> GSHMFSLITWNIDGLDLNNLSERARGVCSYLALYSPDVIFLQEVIPPYYSYLKKRSSNYEIITGHEEGYFTAIMLKKSRVKLKSQEIIPFPSTKMMRNLLCVHVNVSGNELCLMTSHLESTRGHAAERMNQLKMVLKKMQEAPESATVIFAGDTNLRDREVTRSGGLPNNIVDVWEFLGKPKHCQYTWDTQMNSNLGITAACKLRFDRIFFRAAAEEGHIIPRSLDLLGLEKLDCGRFPSDHWGLLCNLDIIL

Tyrosyl-DNA phosphodiesterase 2 (TDP2) {also known as TRAF and TNF receptor-associated gene (TTRAP) or ETS1-associated protein II (EAPII) } is a 5′-tyrosyl DNA phosphodiesterase that can remove the covalently-attached abortive complexes generated by DNA topoisomerase II (TOP2) when it is unable to complete its normal catalytic cycle. Fortunately, this type of DNA lesion is efficiently repaired, in part though the action of TDP2, which hydrolyses the phosphotyrosyl bond in a magnesium cofactor-dependent reaction, leaving ligatable 5′-phosphate moieties. Consequently, TDP2 has attracted interest as a target for small molecule inhibitors that might have utility in overcoming innate or acquired resistance to TOP2 poisons. Using a ‘humanized’ mouse TDP2 expression construct, we have now determined X-ray crystal structures of the catalytic domain of TDP2 in complex with deazaflavin inhibitors, revealing the unusual molecular interactions underpinning their mode of action.

As with the apo-hTDP2CAT crystals, co-crystals with 163 presented severe problems with anisotropy during data collection. Again, multiple crystals were screened before a dataset that could be truncated isotropically, to a maximum resolution of 3.4 Å, was obtained. Despite the low-resolution, which prevents detailed characterization of specific protein-drug interactions, clear difference electron density maps identified the binding site and general pose of this class of inhibitor bound to TDP2. The experimentally determined binding-mode of 163 is surprisingly different from that predicted by molecular docking studies, in which the pyrimido-dione ring of the tricyclic core, was hypothesized to bind to the magnesium cofactor–required for catalytic activity of TDP2–and made few (if any) hydrogen bonds directly to the protein. Instead, our data indicate that the tricyclic deazaflavin core of 163 unexpectedly packs against an extended hydrophobic patch, formed by the side chains of Trp297, Thr299, Leu305, Ile307, Cys311, Leu313 and Phe315, which lies at the mouth of the channel leading to the active site, more than 9 Å from the catalytic Mg2+ ion bound by the carboxyl side chains of Asp122 and Glu152. Significantly, the M7-motif maps to the binding site we observe for 163 in hTDP2CAT, where human TDP2 residues Cys311 and Leu313, along with Ala309, coalesce to form a ‘hydrophobic-shelf’ on which the deazaflavin core of 163 sits. Replacement of Cys311 and Leu313 in hTDP2 with the equivalent residues Tyr321 and His323 in mTDP2 disrupts this hydrophobic-shelf and explains the resistance of the mouse enzyme to the deazaflavin-based inhibitors.> GSMDRRFYGKIVIKGKIKAVTGLHIGSQRDISEIGGIA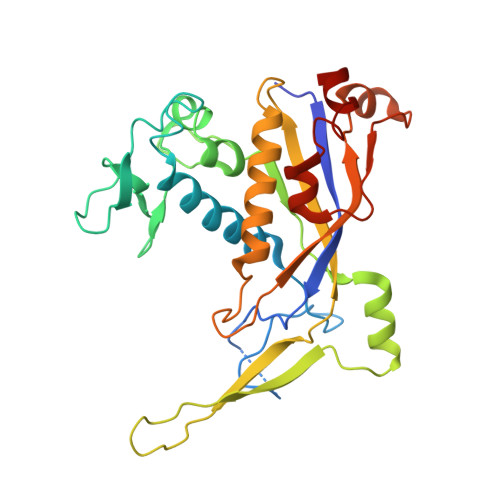NPVIKDPHTGLPYIPGSSLKGRLRSLFEILVNSRLGEWREKYPSLANYSPGSCRPDNQENCGKFFNRKINRGWIHVCPDYETALACPVCRLFGASGKESNFPSRIIVRDAFLTKEWEEKWRAGEAITEAKIEVGIDRVTSQANPRTNERVVAGAEFEFEIIYNVENTTHWRDDIKNLLTAMALLEDSYLGGSGSRGYGKVKFIFDSFEFRPLDYYRTGKDEDIVSIDAREKSVSDILSGFDSLFSEVEGKLEAG>[4x]SNVPHKSSLPEGIRPGTVLRIRGLVPPNASRF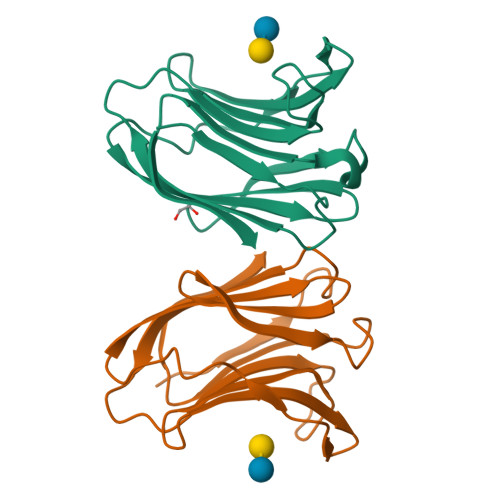HVNLLCGEEQGSDAALHFNPRLDTSEVVFNSKEQGSWGREERGPGVPFQRGQPFEVLIIASDDGFKAVVGAAQYHHFRHRLPLARVRLVEVGGDVQLDSVRIF> DNDSVVEEHGQLSISNGELVNERGEQVQLKGMSSHGLQWYGQFVNYESMKWLRDDWGINVFRAAMYTSSGGYIDDPSVKEKVKEAVEAAIDLDIYVIIDWHILSDNDPNIYKEEAKDFFDEMSELYGDYPNVIYEIANEP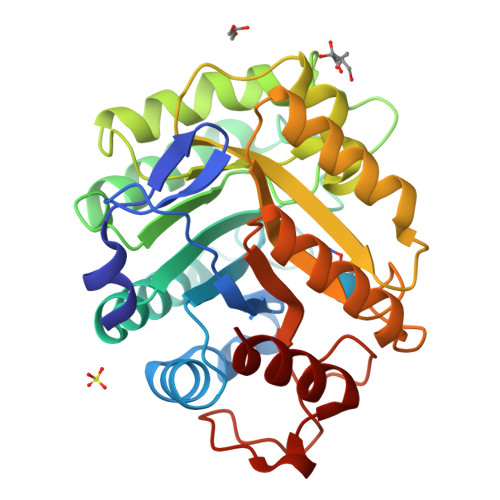NGSDVTWGNQIKPYAEEVIPIIRNNDPNNIIIVGTGTWSQDVHHAADNQLADPNVMYAFHFYAGTHGQNLRDQVDYALDQGAAIFVSEWGTSAATGDGGVFLDEAQVWIDFMDERNLSWANWSLTHKDESSAALMPGANPTGGWTEAELSPSGTFVREKIRES> PISPIETVPVKLKPGMDGPKVKQWPLTEEKIKALVEICTEMEKEGKISKIGPENPYNTPVFAIKKKDSTKWRKLVDFRELNKRTQDFWEVQLGIPHPAGLKKKKSVTVLDVGDAYFSVPLDEDFRKYTAFTIPSINNETPGIRYQYNVLPQGWKGSPAIFQSSMTKILEPFKKQNPDIVIYQYIDDLYVGSDLEIGQHRTKIEELRQHLLRWGLTTPDKKHQKEPPFLWMGYELHPDKWTVQPIVLPEKDSWTVNDIQKLVGKLNWASQIYPGIKVRQLSKLLRGTKALTEVIPLTEEAELELAENREILKEPVHGVYYDPSKDLIAEIQKQGQGQWTYQIYQEPFKNLKTGKYARMRGAHTNDVKQLTEAVQKITTESIVIWGKTPKFKLPIQKETWETWWTEYWQATWIPEWEFVNTPPLVKLWYQLEKEPIVGAETFYVDGAANRETKLGKAGYVTNKGRQKVVPLTNTTNQKTELQAIYLALQDSGLEVNIVTDSQYALGIIQAQPDKSESELVNQIIEQLIKKEKVYLAWVPAHKGIGGNEQVDKLVSAGIRK;> PISPIETVPVKLKPGMDGPKVKQWPLTEEKIKALVEICTEMEKEGKISKIGPENPYNTPVFAIKKKDSTKWRKLVDFRELNKRTQDFWEVQLGIPHPAGLKKKKSVTV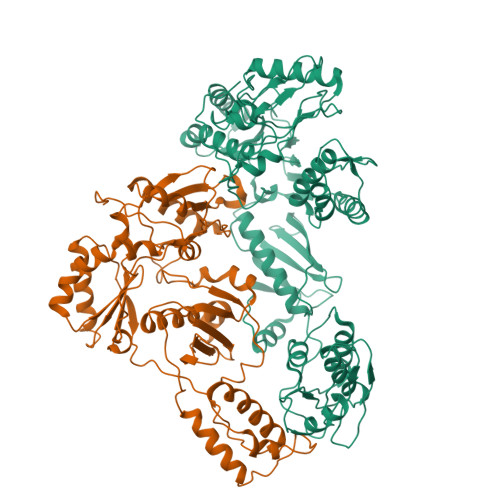LDVGDAYFSVPLDEDFRKYTAFTIPSINNETPGIRYQYNVLPQGWKGSPAIFQSSMTKILEPFKKQNPDIVIYQYIDDLYVGSDLEIGQHRTKIEELRQHLLRWGLTTPDKKHQKEPPFLWMGYELHPDKWTVQPIVLPEKDSWTVNDIQKLVGKLNWASQIYPGIKVRQLSKLLRGTKALTEVIPLTEEAELELAENREILKEPVHGVYYDPSKDLIAEIQKQGQGQWTYQIYQEPFKNLKTGKYARMRGAHTNDVKQLTEAVQKITTESIVIWGKTPKFKLPIQKETWETWWTEYWQATWIPEWEFVNTPPLVKLWY>MHHHHHHHMEQIAQQQPQTLCIKHLAKNYSKRWVVKDVSFEMQSGQIVGLLGPNGAGKTTSFYMVVGLVRMDKGEIHLDNLDLSDLAMHERARKGIGYLPQEASIFRKLTIAENIMAILETRKDLNKQQRQQRLQELLNDFKITHIKDSLGMSVSGGERRRAEIARALAADPKFMLLDEPFAGVDPISVGDIKDIIRNLKDRGIGVLITDHNVRETLAICEHAYIVSEGAVIAEGSPQDILENEQVRKVYLGDDFTV[2x];> MIIRRYLVKQVVSTSLVVIALLTLIMMGGRLIKYFGVAAQGRLDAGVLFSIIGYRMPEFLTLILPLGFFIGLMLVFGRLYVDHEMAVLNGSGISRIRLGQLLIPLALVFLVIQGILMLWMTPWGLRQFDQLSSSQAVRTGFDLVRPKEFISSGPYTIYAGDLSEDRKNLKDIFFYQRAQKEGKPDVMILAKEATRVVMENETANVVDLIQGRRYEIYPGKAKYSQAEFQRYRLRLENDKSATFETDKVEALPSSKLWNKWNDPVIASEMGWRVFGPFTIVIALMMAVALCEVSPRQGRYYRLIPAIFIFASLIVLLIAIRTRISRDELGVWAYPAALAVYGIAAALFSRKQKLAPKIKKQIKRVRA;> MLARRIVAKHVTKTTALAMLGTTIVLVILQVLFTYLGELSNLKADYSAWQAFLYVLWGAPRYLYEILPISALIGAILGLGTLASNSELIVMRSVGISLWRIVGWVIRSALVLVLLSFALSEWVVPYTNERANSVKSHQSVAALGEVRGYWSREGQRFIYVDYANSQGQLKRIQVVDFDDNYRLKSVTNAEQGQFVKDGQWLLNHSQQMAIQGQGDAVLANAAKQPFSLALQPKYVHMVTIDPEDLSFSQLVSFMNYMREYSQVPKTYQLAFWKKVASPFALITLVLVACSFIFGPLRQQSMGFRLVIALFIGLGFYYLQDFLGYASLVYNPSPAWFVLGPIVLMFVAGSYLLYRAR

The impenetrable nature of the outer membrane is due to the presence of a large, amphipathic glycolipid called lipopolysaccharide (LPS) in its outer leaflet. Assembly of the outer membrane requires transport of LPS across a protein bridge that spans from the cytoplasmic membrane to the cell surface. Here, using structural, biochemical and genetic approaches, we show that these antibiotics trap a substrate-bound conformation of the LPS transporter that stalls this machine. The inhibitors accomplish this by recognizing a composite binding site made up of both the Lpt transporter and its LPS substrate.

To assess whether the conformation of LPS in the drug-bound structure reflects an on-pathway intermediate, we solved structures of A. baylyi LptB2FG bound to either E. coli or Acinetobacter LPS but now in the absence of 1. In both cases, the overall conformation and contacts of LPS to the transporter are nearly identical to those determined in the presence of compound 1. These findings are consistent with a mechanism in which compound 1 binds a pre-existing, LPS-loaded state of the transporter complex, identifying this state as a druggable conformation for antibiotic development. Although the specific sequence of events is uncertain, we propose that C-helix movement away from LptFG during the transport cycle permits LPS to bind in the intermediate transport state observed in the structure of the LptB2FG–LPS complex and that this is the state required for inhibitor recognition.>MITAFVLIRPRGNRVQALGEAIAELPQVAEVYSVTGPYDLVALVRLKDVEELDDVVTQGILSLEGVERTETLLAF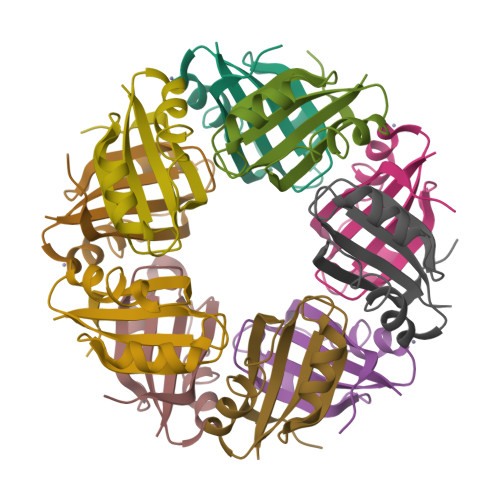RAYPRRLLDQGFALGQG[10x]(2~{R},3~{S},4~{S},5~{R},6~{R})-2-(hydroxymethyl)-6-(5-phenyl-1,2,3,4-tetrazol-2-yl)oxane-3,4,5-triol 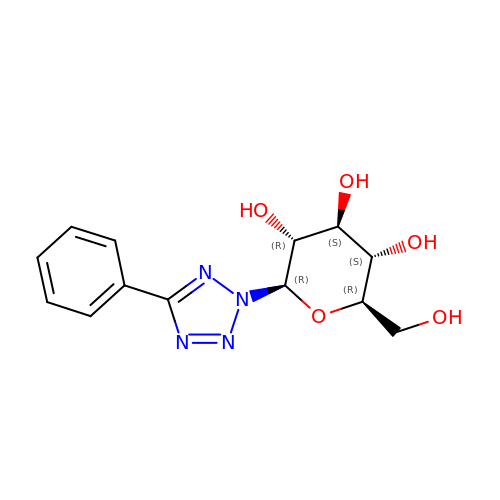| C13 H16 N4 O5 | DNXJDWRGEZLNKO-BZNQNGANSA-N>[2x]MDWVVAPISVPENGKGPFPQRLNQLKSNKDRDTKIFYSITGPGADSPPEGVFAVEKETGWLLLNKPLDREEIAKYELFGHAVSENGASVEDPMNISIIVTDQNDHKPKFTQDTFRG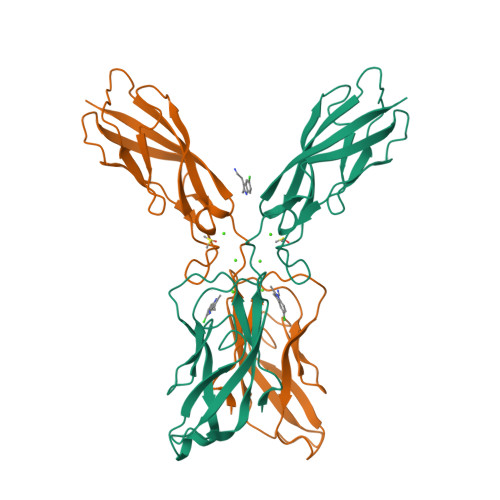SVLEGVLPGTSVMQVTATDEDDAIYTYNGVVAYSIHSQEPKDPHDLMFTIHRSTGTISVISSGLDREKVPEYTLTIQATDMDGDGSTTTAVAVVEILD> MDLNFIQVILVIFVAFLAGVEGILDQFHFHQPVIACTLIGLVTGNLLPCLILGGTLQMIALGWANVGAAVAPDAALASIASAIILVLGGQGKAGVTSAIAIAVPLAVAGLLL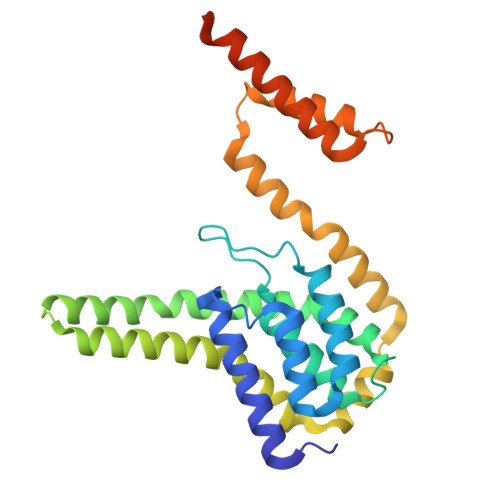TIIVRTLATGIVHIMDAAAKEGNFRKIEMWQYIAIIMQGVRIAIPAGLILAIGAGPVKEMLTAMPVWLTDGLAIGGGMVVAVGYAMVINMMATKEVWPFFAIGFVLATISQLTLIGLGAIGISLALIYLALSKQGSGNNGGGSNTGDPLGDIIDNY alpha-L-gulopyranuronic acid | C6 H10 O7 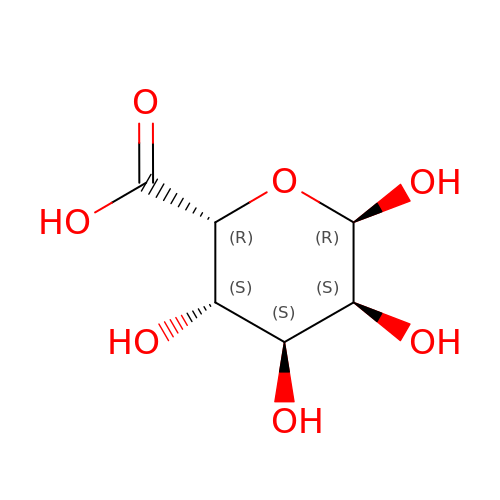| AEMOLEFTQBMNLQ-AZLKCVHYSA-N> GSHMDHLPMPKFGPLAGLRVVFSGIEIAGPFAGQMFAEWGAEVIWIENVAWADTIRVQPNYPQLSRRNLHALSLNIFKDEGREAFLKLMETTDIFIEASKGPAFARRGITDEVLWQHNPKLVIAHLSGFGQYGTEEYTNLPAYNTIAQAFSGYLIQNGDVDQPMPAFPYTADYFSGLTATTAALAALHKVRETGKGESIDIAMYEVMLRMGQYFMMDYFNGGEMCPRMSKGKDPYYAGCGLYKCADGYIVMELVGITQIEECFKDIGLAHLLGTPEIPEGTQLIHRIECPYGPLVEEKLDAWLATHTIAEVKERFAELNIACAKVLTVPELESNPQYVARE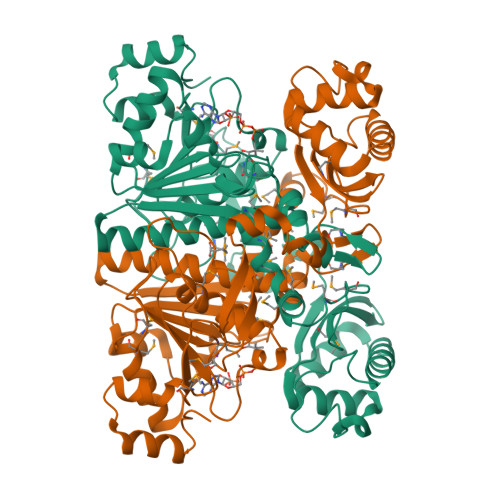SITQWQTMDGRTCKGPNIMPKFKNNPGQIWRGMPSHGMDTAAILKNIGYSENDIQELVSKGLAKVED Here we describe the three-dimensional structure and mechanistic characterization of the enzyme encoded by susB, a GH97 α-glucosidase from B. thetaiotaomicron (BtGH97a). BtGH97a was shown to hydrolyze a range of substrate sizes from maltose to maltoheptaose, and both α-1,4 and α-1,6 linkages. The tertiary structure of BtGH97a reveals three domains; an N-terminal β-super-sandwich domain (residues 1–317), followed by a canonical (β/α)8 barrel (residues 318–636) and a C-terminal β sheet domain (residues 637–738). The three-dimensional structure and kinetic analyses of BtGH97a reveal an unusual calcium ion-dependent catalytic center in which a glutamate residue is poised to activate the nucleophilic water molecule with both general acid and calcium ion assistance to leaving group departure.

The structure of BtGH97a was solved using X-ray crystallography data to 1.90 Å resolution. Phasing was performed using single-wavelength anomalous dispersion data collected at the peak wavelength (0.9795 Å) for selenium, and the majority of the protein was built automatically. A calcium ion is present in the (β/α)8 barrel domain; it is octahedrally coordinated by four glutamate residues (Glu194, Glu508, Glu526, and Glu532) and both oxygen atoms of a molecule of ethylene glycol, which was sequestered from the cryoprotectant. The calcium ions in each molecule of the asymmetric unit in the native structure (and the complexes described below) yield atomic B factors of 14–16 Å2 when refined with unitary occupancy. Superposition with other (β/α)8 barrel GHs (data not shown), as well as the presence of the four glutamates, suggests that the calcium ion is, in fact, bound in the active-site region of the enzyme. The calcium ion displays high apparent affinity and may only partially be removed using EDTA or Chelex. Partial removal of the calcium causes a substantial reduction in activity, but the enzyme maintains a residual activity, confirming high metal ion affinity. The addition of calcium to the EDTA-treated enzyme resulted in restoration of full activity; all further kinetics experiments were thus conducted in the presence of 10 mM CaCl2, at which the enzyme had full activity.

>[2x]MGSSHHHHHHQQKLTSPDNNLVMTFQVDSKGAPTYELTYKNKVVIKPSTLGLELKKEDNTRTDFDWVDRRDLTKLDSKTNLYDGFEVKDTQTATFDETWQPVWGEEKEIRNHYNELAVTLYQPMNDRSIVIRFRLFNDGLGFRYEFPQQKSLNYFVIKEEHSQFGMNGDHIAFWIPGDYDTQEYDYTISRLSEIRGLMKEAITPNSSQTPFSQTGVQTALMMKTDDGLYINLHEAALVDYSCMHLNLDDKNMVFESWLTPDAKGDKGYMQTPCNTPWRTIIVSDDARNILASRITLNLNEPCKIADAASWVKPVKYIGVWWDMITGKGSWAYTDELTSVKLGETDYSKTKPNGKHSANTANVKRYIDFAAAHGFDAVLVEGWNEGWEDWFGNSKDYVFDFVTPYPDFDVKEIHRYAARKGIKMMMHHETSASVRNYERHMDKAYQFMADNGYNSVKSGYVGNIIPRGEHHYGQWMNNHYLYAVKKAADYKIMVNAHEATRPTGICRTYPNLIGNESARGTEYESFGGNKVYHTTILPFTRLVGGPMDYTPGIFETHCNKMNPANNSQVRSTIARQLALYVTMYSPLQMAADIPENYERFMDAFQFIKDVALDWDETNYLEAEPGEYITIARKAKDTDDWYVGCTAGENGHTSKLVFDFLTPGKQYIATVYADAKDADWKENPQAYTIKKGILTNKSKLNLHAANGGGYAISIKEVKDKSEAKGLKRL>MKYVVVSGGVISGIGKGVLASSTGMLMKTLGLKVTSIKIDPYMNIDAGTMSPLEHGECFVLDDGGETDLDLGNYERYLGVTLTKDHNITTGKIYSHVIAKERKGDYLGKTVQIVPHLTNAIQDWIERVAKIPVDDTGMEPDVCIIELGGTVGDIESAPFVEALRQFQFKVGKENFALIHVSLVPVIHGEQKTKPTQAAIKGLRSLGLVPDMIACRCSETLDKPTIDKIAMFCHVGPEQVVNVHDVNSTYHVPLLLLEQKMIDYLHARLKLDEISLTEEEELLSKWKATTGNFDETVKIALVGKYTNLKDSYLSVIKALEHSSMKCRRKLDIKWVEATDLEPEAQESNKTKFREAWNMVSTADGILIPGGFGVRGTEGMVLAARWARENHIPFLGVCLGLQIATIEFTRSVLGRKDSHSAEFYPDIDEKNHVVVFMMRLGLRPTFFQNETEWSQIKKLYGDVSEVHERHRHRYEINPKMVDELENNGLIFVGKDDTGKRCEILELKNHP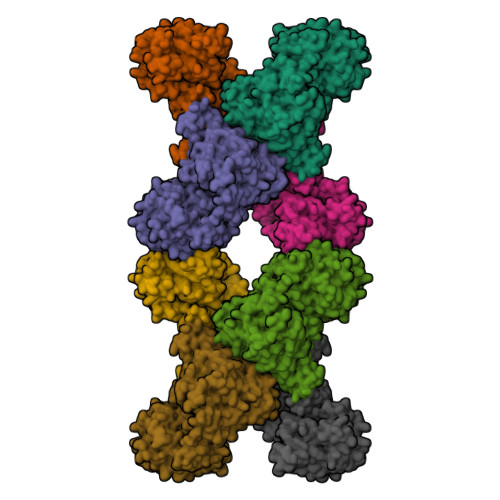YYIATQYHPEYTSKVLDPSKPFLGLVAASAGILQDVIEGKYDLEA[8x]Here we present the structural and functional studies of SCARB2, a functional receptor of the important human enterovirus 71 (EV71). SCARB2 is responsible for attachment as well as uncoating of EV71. SCARB2 is ubiquitously expressed and serves as a common receptor for all clinically isolated EV71 strains, CVA16, CVA7 and CVA14. SCARB2 (residues 37–430) consists of three domains arranged in a “Kidney” shape.

To gain an understanding of the molecular basis of SCARB2-mediated uncoating of EV71 under acidic conditions, we solved the crystal structures of the ectodomain of SCARB2 under both neutral (pH 7.5) (hereafter denoted as nSCARB2) and acidic conditions (pH 4.8) (hereafter denoted as aSCARB2). A striking difference in the position of the “cap” is observed between structures at acidic and neutral pH. In contrast, at pH 7.5, the re-positioning of α5 in vicinity of α4 and α7 blocks the membrane-distal end of the tunnel, decreasing its void volume from 4,867 Å3 to 4,554 Å3 [calculated by program HOLLOW]. Thus in nSCARB2, α5 (residues 157–164) adopts a short helical conformation. Helices α4, α5 and α7 are held together in a compact cluster by hydrophobic interactions involving residues W146, L152, I156, Y163 of α4–α5 and I184, L187, I188, F191, I195 from α7. Under neutral conditions, a cap closes the entrance of the lipid-transfer tunnel of SCARB2. Amongst these multiple sites, based on the contour of the electron density and prior knowledge that lysosomal enzymes are often modified with Man9GlcNA2-P, the glycan at N325 of nSCARB2 was modeled as Man8GlcNA2. N325 is located at the bottom of a cleft formed between helices α11 and α12. Man8GlcNA2 protrudes to the surface out of this chasm and stations itself in vicinity of the cap. Notably, the sugar moieties adjacent to α4 and α5 are stabilized by P314, E145 and H150.

>[2x]IEKKIVLRNGTEAFDSWEKPPLPVYTQFYFFNVTNPEEILRGETPRVEEVGPYTYRELRNKANIQFGDNGTTISAVSNKAYVFERDQSVGDPKIDLIRTLNIPVLTVIEWSQVHFLREIIEAMLKAYQQKLFVTHTVDELLWGYKDEILSLIHVFRPDISPYFGLFYEKNGTNDGDYVFLTGEDSYLNFTKIVEWNGKTSLDWWITDKCNMINGTDGDSFHPLITKDEVLYVFPSDFCRSVYITFSDYESVQGLPAFRYKVPAEILANTSDNAGFCIPEGNCLGSGVLNVSICKNGAPIIMSFPHFYQADERFVSAIEGMHPNQEDHETFVDINPLTGIILKAAKRFQINIYVKKLDDFVETGDIRTMVFPVMYLNESVHIDKETASRLKSMIN>[2x]RPEKPVYLSVKADNSMFIGNDPVTDETMITALNALTEGKKDTTIFFRADKTVDYETLMKVMDTLHQAGYLKIGLVGEETAKAK;> QPISVTMVT

Gram-negative bacteria use TonB-dependent transport to take up nutrients from the external environment, employing the Ton complex to import a variety of nutrients that are either scarce or too large to cross the outer membrane unaided. The Ton complex contains an inner-membrane motor (ExbBD) that generates force, as well as nutrient-specific transport proteins on the outer membrane. These two components are coupled by TonB, which transmits the force from the inner to the outer membrane. Here, we identify a conserved motif within TonB that we term the D-box, which serves as an attachment point for ExbD.

The ExbD periplasmic domain alone yielded no crystals, even when high concentrations of protein were used (data not shown); however, crystals were readily obtained when the periplasmic domain was mixed with the D-box peptide. Two different crystal forms were obtained, both diffracting to approximately 1.4 Å; in each, the asymmetric unit comprises a 2:1 ExbD:D-box complex. Essentially identical structures are seen for the complex in two different crystal forms; in addition, these structures are highly similar to one recently published, which describes a 2:1 complex of the ExbD periplasmic domain with a 23-mer TonB peptide that includes the D-box sequence. Each ExbD monomer contains a five-stranded sheet, with two helices packed against one face of that sheet; two ExbD monomers assemble into a dimer with approximate two-fold symmetry. The two protomers contact one another via the loops connecting strand three and helix 2, imparting a V-shape to the dimer, with a deep groove between the two halves. The D-box peptide binds within this groove and, as hypothesized, assumes an extended conformation, forming a strand that is recruited to the edges of the beta sheets of both ExbD monomers. Residues 60 to 62 of the peptide interact with residues 130 to 134 of one ExbD chain (Chain A), forming a parallel pattern of inter-strand hydrogen bonds, while residues 57 to 59 of the peptide interact with residues 130 to 132 of the other ExbD chain (Chain B), forming an anti-parallel hydrogen-bonding pattern. Thus, a single D-box strand is simultaneously recruited to the edges of two different beta sheets, one from each of the ExbD protomers. In particular, the side chains of Ile-57, Val-59, and Met-61 all point downward and are captured within hydrophobic cavities formed in the cleft between the two ExbD protomers. Met-61 lies at the C-terminal end of the D-box, and the hydrophobic pocket containing its side chain is partially formed by the side chain of Leu-132, offering an explanation for why the L132Q mutant fails to bind the D-box.>[2x]MAS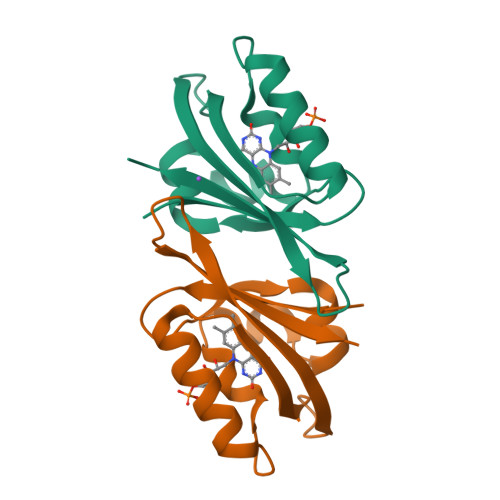GMIVTDAGADQPIVFVNRAFSTITGYAPNEVLGRNARFLQGPQTDAATVARLREAIAAARPIQERILNYRKDGQPFWNQLSISPVRDETGNVVAFVGVRTDVTAHHHHHH>PYITVGRHLDFLRPGLRFGGSQSSKYTYYTVEVKIDTVNLPLYKDSRSLDPHVTGTFTIKNLTPVLDKVVTLFEGYVINYNQFPLCSLHWPAEETLDPYMAQRESDCSHWKRFGHFGSDNWSLTERNFGQYNHESAEFMNQR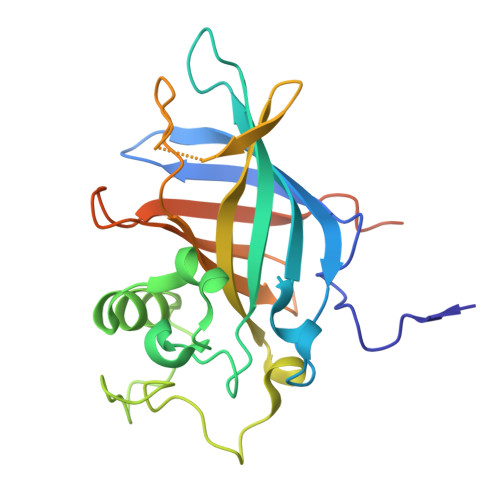YIYLKWKERFLLDDEEQENLMLDDNHHLEGASFEGFYYVCLDQLTGSVEGYYYHPACELFQKLELVPTNCDALNTYSSGFEIALEHHHHHHHH[2x]>MQNITQSWFVQGMIKATTDAWLKGWDERNGGNLTLRLDDADIAPYHDNFHQQPRYIPLSQPMPLLANTPF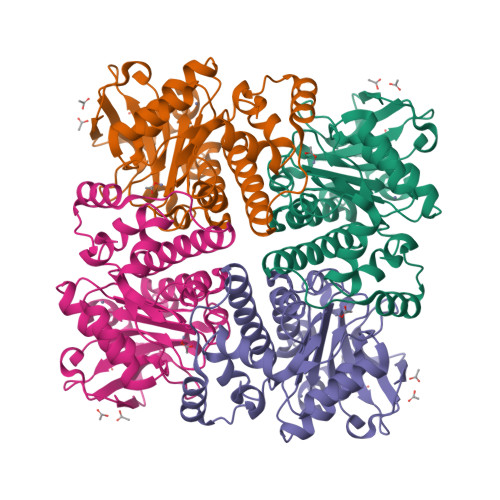IVTGSGKFFRNVQLDPAANLGIVKVDSDGAGYHILWGLTNEAVPTSELPAHFLSHCERIKATNGKDRVIMHCHATNLIALTYVLENDTAVFTRQLWEGSTECLVVFPDGVGILPWMVPGTDAIGQATAQEMQKHSLVLWPFHGVFGSGPTLDETFGLIDTAEKSAQVLVKVYSMGGMWQTISREELIALGKRFGVTPLASALSL[2x]> GAMAAPAACTRFSDNYDIKEELGKG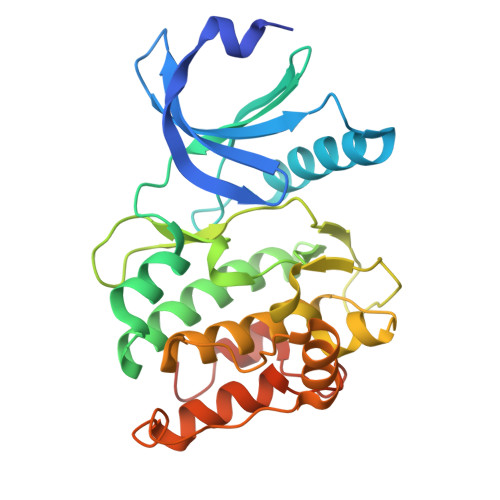AFSIVKRCVQKSTGFEFAAKIINTKKLTARDFQKLEREARICRKLHHPNIVRLHDSIQEENYHYLVFDLVTGGELFEDIVAREFYSEADASHCIQQILESVNHCHQNGVVHRNLKPENLLLASKAKGAAVKLADFGLAIEVQGDHQAWFGFAGTPGYLSPEVLKKEPYGKSVDIWACGVILYILLVGYPPFWDEDQHRLYSQIKAGAYDYPSPEWDTVTPEAKNLINQMLTVNPNKRITAAEALKHPWICQRERVASVVH> TTIVSVRRNGQVVVGGDGQVSLGNTVMKGNARKVRRLYNGKVLAGFAGGTADAFTLFELFERKLEMHQGHLLKSAVELAKDWRTDRALRKLEAMLIVADEKESLIITGIGDV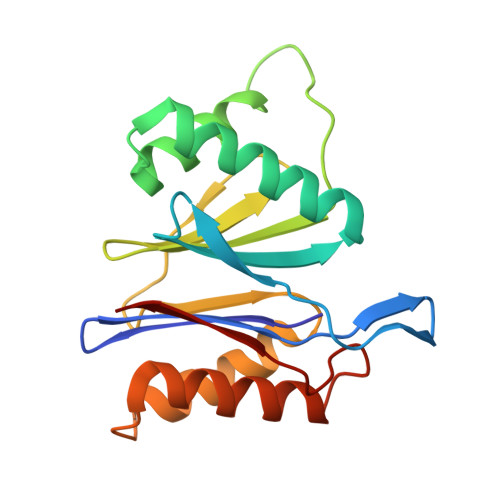VQPEEDQILAIGSGGNYALSAARALVENTELSAHEIVEKSLRIAGDICVFTNTNFTIEELPN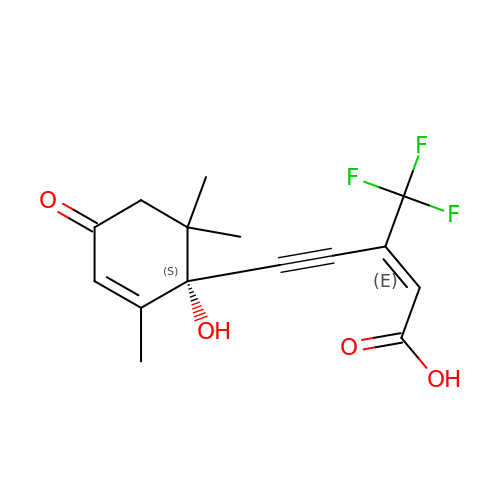(~{E})-3-(trifluoromethyl)-5-[(1~{S})-2,6,6-trimethyl-1-oxidanyl-4-oxidanylidene-cyclohex-2-en-1-yl]pent-2-en-4-ynoic acid | C15 H15 F3 O4 | CQNKVZZCXKPIPC-DNGMOHDESA-N(1~{R},3~{S},5~{Z})-5-[(2~{E})-2-[(1~{R},3~{a}~{S},7~{a}~{R})-7~{a}-methyl-1-[(1~{S})-1-[(2~{S},5~{R})-5-(2-oxidanylpropan-2-yl)oxolan-2-yl]ethyl]-2,3,3~{a},5,6,7-hexahydro-1~{H}-inden-4-ylidene]ethylidene]-4-methylidene-cyclohexane-1,3-diol 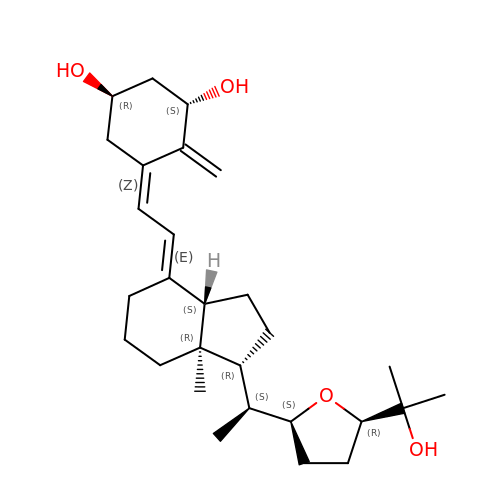| C28 H44 O4 | DDIWZQGTNVZJGO-XOJGNBOJSA-N>[8x]SNAMSGMRFGTRLVHGGRRPSAGTGDVVPPIHVSTTYERRAQDEPRYFYGRGENPTREELEECLAGLERAPFATVFSSGQAAAATLLSLVRPGQCVVSTDDVYAGTDGLFDLAARQGVRVRYADLTTPEG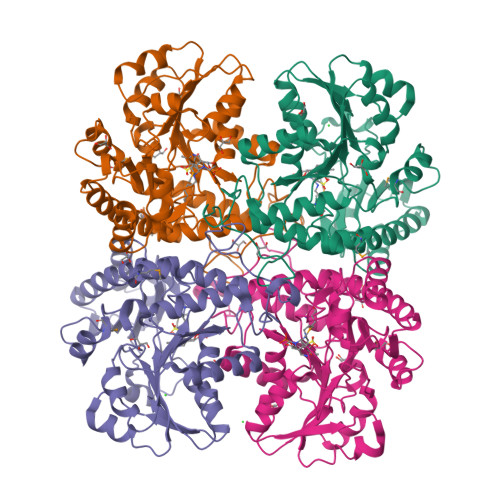IAAALAEPDLALVWIETPTNPLLTVVDVAEVSRRAHERGARVVVDNTFASPVLQQPLALGADVSLYSTTKSIAGHADVLGGALVYRDADLHAAVRAYRTTAGNVPGALDCFLVRRGLHTLSLRVHRQVATARVLVERLRASPVVGAVHYPGLPEHPQHAVVKAQMSAPGAIVSFDYLGGPAERLLDRFTLFTCGVSLGGVHSLVECPALMTHRPLSAEARARRGIGESLIRLSVGIEDPQDLAEDLSRALAGGT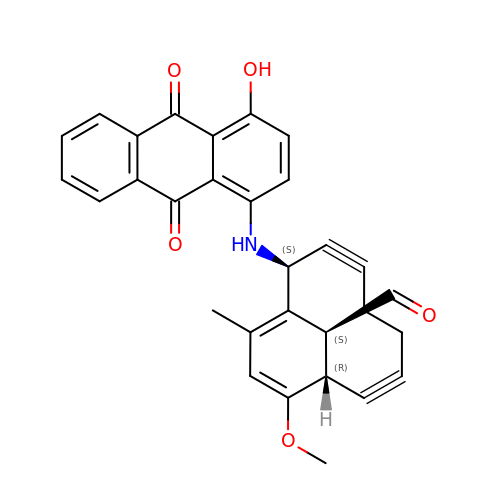(1R,8S,13S)-8-[(4-hydroxy-9,10-dioxo-9,10-dihydroanthracen-1-yl)amino]-12-methoxy-10-methylbicyclo[7.3.1]trideca-9,11-diene-2,6-diyne-13-carbaldehyde | C30 H23 N O5 | NLNOIBOHBHXKKN-NYVOZVTQSA-N1-[6-(2-hydroxypropan-2-yl)pyridin-2-yl]-6-{[4-(4-methylpiperazin-1-yl)phenyl]amino}-2-(prop-2-en-1-yl)-1,2-dihydro-3H-pyrazolo[3,4-d]pyrimidin-3-one 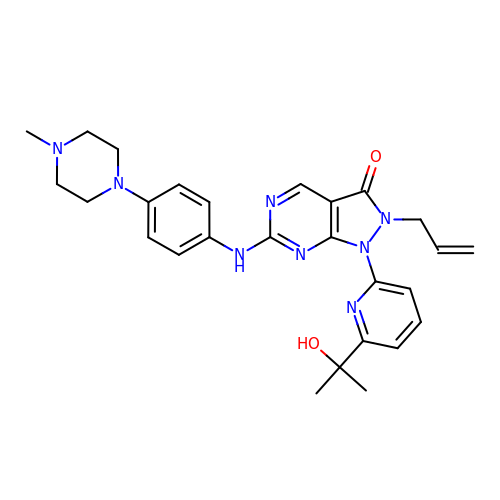| C27 H32 N8 O2 | BKWJAKQVGHWELA-UHFFFAOYSA-N>ATMQPFHSPEESVNSQFYLPPPPGNDDPAFRYDKEAYFKGYAIKGSPRWKQAAEDADISVENIARIFSPVVGAKINPKDTPETWNMLQNLLKMGGYYATASAKKYYMRTRPFVLFNHSTCRPEDENTLRKDGSYPSGHDAYSTLLALVLSQARPERAQELARRGWEFGQSRVICGAHWQSDVDAGRYVGAVEFARLQTIPAFQKSLAKVREELNDKNNLLSKEERPELN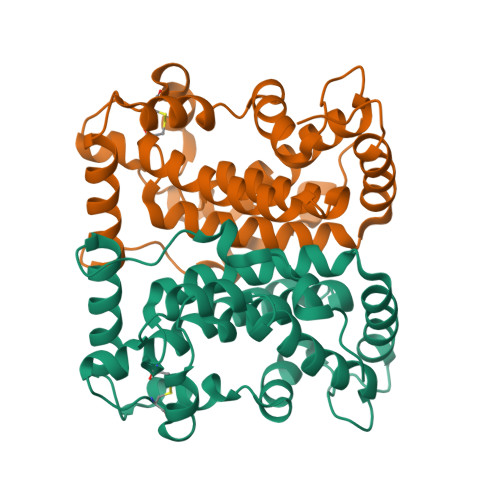Y[4x]Here we introduce RFpeptides, a denoising diffusion-based pipeline for designing macrocyclic binders against protein targets of interest. We tested 20 or fewer designed macrocycles against each of four diverse proteins and obtained binders with medium to high affinity against all targets. X-ray structures for macrocycle-bound myeloid cell leukemia 1, γ-aminobutyric acid type A receptor-associated protein and RbtA complexes match closely with the computational models, with a Cα root-mean-square deviation < 1.5 Å to the design models. RFpeptides is not limited to generating macrocycles with particular motifs or topologies; the diffusion process generates macrocycles with diverse shapes and sizes and selects the topologies appropriate for the protein being targeted. Among the four targets tested here, binders for MCL1 and MDM2 have helical motifs, binders for GABARAP have a β-sheet topology and binders for RbtA sample looplike conformations that make extensive contacts with the flat surface of this target.

We designed macrocycles against Rhombotarget A (RbtA), a recently identified cell surface protein from the ESKAPE pathogen, Acinetobacter baumannii. On the basis of our preliminary design runs without hotspots to guide the diffusion, we identified a patch in the N-terminal domain to pursue in our large-scale design calculations against this target and defined hotspots Leu144, Phe202, Phe204, Tyr206, Val208, Leu231 and Ala269 for peptide backbone generation. In contrast to the concave pockets targeted for MDM2 and MCL1, this selected patch for RbtA is considerably flatter and difficult to target with conventional computational and experimental approaches. On the basis of further binding experiments with SPR, we determined the dissociation constant (Kd) of the best binder, RBB_D10, to be 9.4 nM. To confirm the structures of RbtA and RBB_D10 and the binding mode between them, we determined the high-resolution X-ray crystal structure of apo and macrocycle-bound RbtA using X-ray crystallography at 2 Å and 2.6 Å resolution, respectively. The complex structure also confirmed the structure and binding mode of our designed macrocycle, RBB_D10, with the X-ray structure matching the design model with an r.m.s.d. of 1.4 Å. Notably, the conformation adopted by the macrocycle in the X-ray structure, including the side-chain rotamers involved in interactions with the target, was almost identical to the design model with an r.m.s.d. of 0.4 Å. Together, these data highlight the high accuracy and success rates provided by RFpeptides even while designing macrocycles against targets without deep pockets or targets with no known structures.

>[2x]MGADIEVTTTIDEDVDNTVCSLREAVELINKRNSSDSTVVASVKDGYHGCGNKDASSNIILQRDKEYTLNSRITITAPLTISTAKNDSTLVDTDQPGSHNATIKMAGTDQLFKIDDESVEKASFSVLLSDLNLQGAGANSKVLTGGLILNHEKLTIQNSRLTGGYANQGGVIYNQGFASKSDRTFGFVYIVNSLIQNNKAAQGGVIYSEQPLFLITQSVIRDNEVSNTSGSLFFSQDSFDDESTGEYVVQRAIGLSNSTVFHNKGGFITNVRDGMFVNNITMIKNDKGLFLEAPQGNASISNSILVGNTINCQANSTDKAIIQSNLVTTECNRNASVKVPNILYPANQKLIAGSTDEGVCDVASKDGLLCPFNTPKDSFLGFFKPRLLESYNTLADSLIINKGRLYSDGTSVGLASCETLDQRGKRRTGYDELCDLGAIEYIGLNDIFEAQKIEWHELEHHHHHH;>[2x]KLFGPDPYLPENVQ>[3x]MRTGQQYLESLRDGRQVYVGGELIDDVTTHPKTSGYAKAIAEYYDLHLDPEHQDVLTFVDDDGVRKSMHWFLPRSKADAARRRAYHEFWFRHFQGGIFTRPPAGMHVVMYAQIDDPEPWGDNAVVAGGRTISFADNIRSQWQRVTTDDVALSPMFVDVQFDRGRDDALVETPMLSIVEQNDQGIVVRGWKAMGTSLPFVNELLVGNLWRPGQTSDQTVYAIVPVNTPGLSLVCRQSNATPDADPYDHPLSTIGDELDGMAYFDDVFIPWENVQHIGNPDHAKWYPQRQFDWVHIETQIRHAVHAELIVGLALLLTNALGTNNNPIVQSQLADLVRFRETCKAFAIAAEETGFTTAGGLFKPNNIYVDLGRAHYLENIHNAVNQLIEFCGRGVVMSPTKADFDHPFLGPKLEEALRGTSISARDRVSIFRQISERYLTQWGARHEMFEKFNGTPLYLV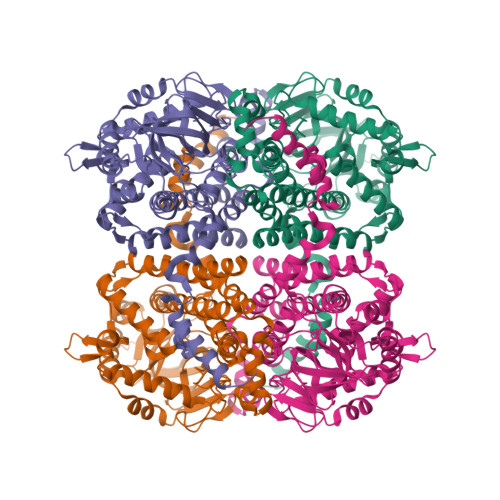RLLTMQRTEYQVDGPLTDLARQVLGFGDTEALAARAAEVEKNSNWASVAYQPEYAREQDVRDGYYKETEKVLEHHHHHH>EERPYAYVKISDGCDRGCTFCSIPSFKGSLRSRSIEDITREVED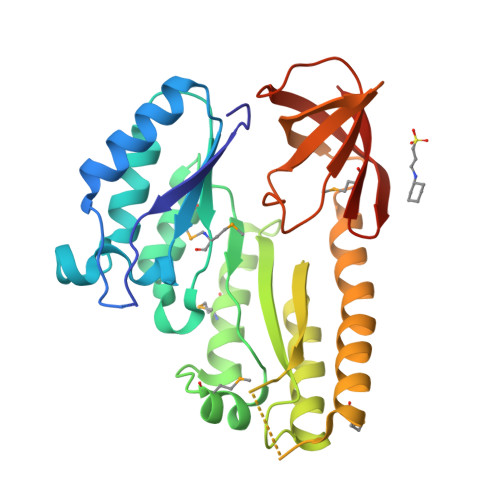LLKEGKKEIILVAQDTTSYGIDLYRKQALPDLLRRLNSLNGEFWIRVMYLHPDHLTEEIISAMLELDKVVKYFDVPVQHGSDKILKLMGRTKSSEELKKMLSSIRERFPDAVLRTSIIVGFPGETEEDFEELKQFVEEIQFDKLGAFVYSDEEGTVAFNLKEKVDPEMAKRRQEELLLLQAEISNSRLDRFVGKKLKFLVEGKEGKFLVGRTWTEAPEVDGVVFVRGKGKIGDFLEVVIKEHDEYDMWGSVILEHHHHHH[8x]> GGAUCUUCGGGGCA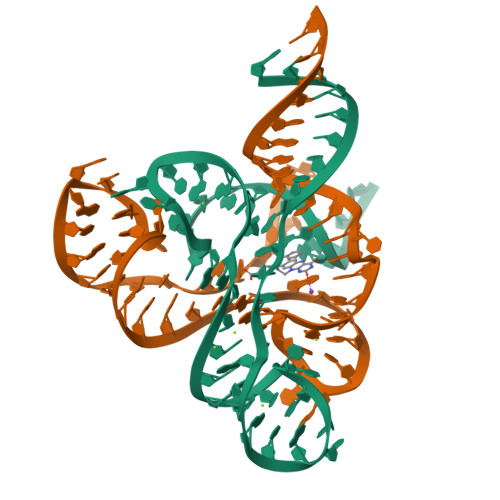GGGUGAAAUUCCCGACCGGUGGUAUAGUCCACGAAAGCUU;> GCUUUGAUUUGGUGAAAUUCCAAAACCGACAGUAGAGUCUGGAUGAGAGAAGAUUC> ETGMPQYST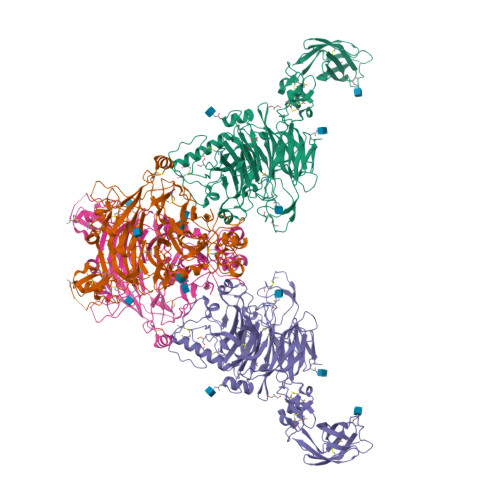FHSENRDWTFNHLTVHRRTGAVYVGAINRVYKLTGNLTIQVAHKTGPEEDNKACYPPLIVQPCSEVLTLTNNVNKLLIIDYSENRLLACGSLYQGVCKLLRLDDLFILVEPSHKKEHYLSSVNKTGTMYGVIVRSEGEDGKLFIGTAVDGKQDYFPTLSSRKLPRDPESSAMLDYELHSDFVSSLIKIPSDTLALVSHFDIFYIYGFASGGFVYFLTVQPETPDGMAINSAGDLFYTSRIVRLCKDDPKFHSYVSLPFGCTRAGVEYRLLQAAYLAKPGEALAQAFNISSDEDVLFAIFSKGQKQYHHPPDDSALCAFPIRAINLQIKERLQSCYHGEGNLELNWLLGKDVQCTKAPVPIDDNFCGLDINQPLGGSTPVEGLTLYTTSRDRLTSVASYVYNGYSVVFVGTKSGKLKKIRADGPPHGGVQYEMVSVFKDGSPILRDMAFSINQLYLYVMSERQVTRVPVESCEQYTTCGECLSSGDPHCGWCALHNMCSRRDKCQRAWEANRFAASISQCMSLEVHPNSISVSDHSRLLSLVVNDAPNLSEGIACAFGNLTEVEGQVSGSQVICISPGPKDVPVIPLDQDWFGLELQLRSKETGKIFVSTEFKFYNCSAHQLCLSCVNSAFRCHWCKYRNLCTHDPTTCSFQEGRINVSEDCPQGTKHHHHHH;> ETGGFPEDSEPISISHGNYTKQYPVFVGHKPGRNTTQRHRLDIQMIMIMNRTLYVAARDHIYTVDIDTSHTEEIYCSKKLTWKSRQADVDTCRMKGKHKDECHNFIKVLLKKNDDTLFVCGTNAFNPSCRNYRVDTLETFGDEFSGMARCPYDAKHANIALFADGKLYSATVTDFLAIDAVIYRSLGDSPTLRTVKHDSKWLKEPYFVQAVDYGDYIYFFFREIAVEYNTMGKVVFPRVAQVCKNDMGGSQRVLEKQWTSFLKARLNCSVPGDSHFYFNILQAVTDVIRINGRDVVLATFSTPYNSIPGSAVCAYDMLDIANVFTGRFKEQKSPDSTWTPVPDERVPKPRPGCCAGSSSLEKYATSNEFPDDTLNFIKTHPLMDEAVPSIINRPWFLRTMVRYRLTKIAVDNAAGPYQNHTVVFLGSEKGIILKFLARIGSSGFLNGSLFLEEMNVYNPEKCSYDGVEDKRIMGMQLDRASGSLYVAFSTCVIKVPLGRCERHGKCKKTCIASRDPYCGWVRESGSCAHLSPLSRLTFEQDIERGNTDGLGDCHNSGTKHHHHHH> SNHHRGLASANVDFAFSLYKHLVALSPKKNIFISPVSISMALAMLSLGTCGHTRAQLLQGLGFNLTERSETEIHQGFQHLHQLFAKSDTCLEMTMGNALFLDGSLELLESFSADIKHYYESEVLAMNFQDWATASRQINSYVKNKTQGKIVDLFSGLDSPAILVLVNYIFFKGTWTQPFDLASTREENFYVDETTVVK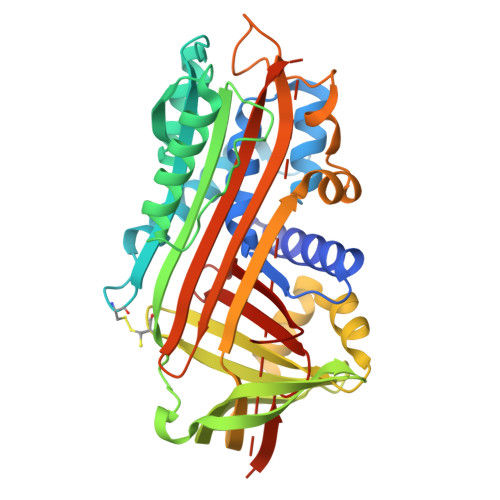VPMMLQSSTISYLHDSELPCQLVQMNYCGNGTVFFILPDKGKMNTVIAALSRDTINRWSAGLTSSQVDLYIPKVTISGVYDLGDVLEEMGIADLFTNQANFSRITQDAQLKSSKVVHKAVLQLNEEGVDTAGSTGVTLNLRSKPIILRFNQPFIIMIFDHFTWSSLFLARVMNPV> MASEQEAIPPLLLRYQDAYEYQRSYGPLIKLEADYDKQLKESQALEHISVSWSLALNNRHLASFTLSTFESNELKVAIGDEMILWYSGMQHPDWEGRGYIVRLPNSFQDTFTLELKPSKTPPPTHLTTGFTAEFIWKGTSYDRMQDALKKFAIDKKSISGYLYYKILGHQVVDISFDVPLPKEFSIPNFAQLNSSQSNAVSHVLQRPLSLIQGPPGTGKTVTSATIVYHLSKIHKDRILVCAPSNVAVDHLAAKLRDLGLKVVRLTAKSREDVESSVSNLALHNLVGRGAKGELKNLLKLKDEVGELSASDTKRFVKLVRKTEAEILNKADVVCCTCVGAGDKRLDTKFRTVLIDESTQASEPECLIPIVKGAKQVILVGDHQQLGPVILERKAADAGLKQSLFERLISLGHVPIRLEVQYRMNPYLSEFPSNMFYEGSLQNGVTIEQRTVPNSKFPWPIRGIPMMFWANYGREEISANGTSFLNRIEAMNCERIITKLFRDGVKPEQIGVITPYEGQRAYILQYMQMNGSLDKDLYIKVEVASVDAFQGREKDYIILSCVRANEQQAIGFLRDPRRLNVGLTRAKYGLVILGNPRSLARNTLWNHLLIHFREKGCLVEGTLDNLQLCTVQLVRHHHHHH;> GPGSTQYNFIIDASAFEKGLGNIKRWCSDCTEAVTLNFYIPTFTLNELDFLQQRRKSFAARESLKFIDRLDDSKFANLKVFIEFPEVLDIILWSDVMEHNDSSGKINIAKLPKRLKNLLKSCIYKCYLEGNEGLHWFLISEDPQIREMAMQCNIPSCSIVDVDSILSKDMNDKSFRESEKFNNMMLKNGTKEESENGREIIRTNFNKTVYASRGTGELWSP

Among these, the nonsense-mediated mRNA decay (NMD) pathway is responsible for the rapid detection and degradation of translated mRNAs harboring premature termination codons (PTCs), which can arise from mutations, transcription, or processing errors as well as alternative or defective splicing events. UPF1 is made of 2 structured domains: a CH-domain known to interact with UPF2 and an ATP-dependent RNA helicase domain (HD). Nmd4 is composed of a PIN domain (for PilT N-terminus) and interacts directly with the helicase domain of Upf1. Nmd4 stimulates Upf1-HD ATPase activity and strengthens Upf1-HD binding to RNA.

Here, we describe the crystal structure of the complex formed between Nmd4 and the Upf1 helicase domain of S. cerevisiae. We tried to crystallize this complex in the absence or presence of a short RNA oligonucleotide, but only obtained crystals of the complex in the absence of RNA. The crystal structure of this complex was solved to 2.4 Å resolution. In the Nmd4/Upf1-HD complex, Upf1-HD adopts a conformation similar to that of human UPF1-HD bound to UPF2 or ADP and phosphate, with the largest difference observed in the orientation of domain 1B (rotation of this domain by 17 to 19° relative to the RecA1 domain in both cases; ). The Nmd4 protein is composed of 2 domains. Second, a C-terminal region (hereafter referred to as the « arm »; residues 168 to 218) folds into a long α-helix (⍺9) followed by a two-stranded antiparallel β-sheet (strands β6 and β7) and a long unstructured region (residues 202 to 218) to embrace Upf1-HD. In total, 39 residues of Nmd4 interact with 44 residues located in the RecA1 domain and in the stalk of Upf1-HD to form an interface area of 2,050 Å2. As a result, a parallel β-zipper is formed between strand β7 of Nmd4 and strand β8 of Upf1 at the interface, generating a three-stranded β-sheet common to the RecA1 domain of Upf1 and the « arm » of Nmd4. The side chain of R210 forms 3 hydrogen bonds with the carbonyl group of F368 as well as with the hydroxyl group of S374 from Upf1-HD, while the W216 side chain stacks on the helix α1 and in particular on G243 of the Upf1-HD stalk region. In conclusion, our crystal structure reveals that Nmd4 interacts primarily with 2 structurally important domains of Upf1-HD, namely the RecA1 and stalk domains, and to a lesser extent with the RecA2 domain.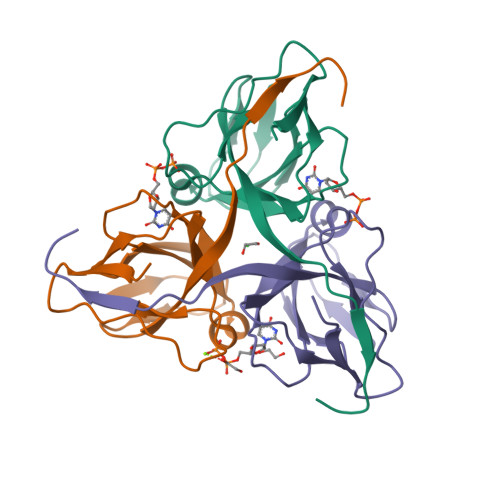>MFNMNINSPVRFVKETNRAKSPTRQSPGAAGYDLYSAYDYTIPPGERQLIKTDISMSMPKFCYGRIAPRSGLSLKGIDIGGGVIDEDYRGNIGVILINNGKCTFNVNTGDRIAQLIYQRIYYPELEEVQSLDSTNRGDQGFGSTGLR[3x]>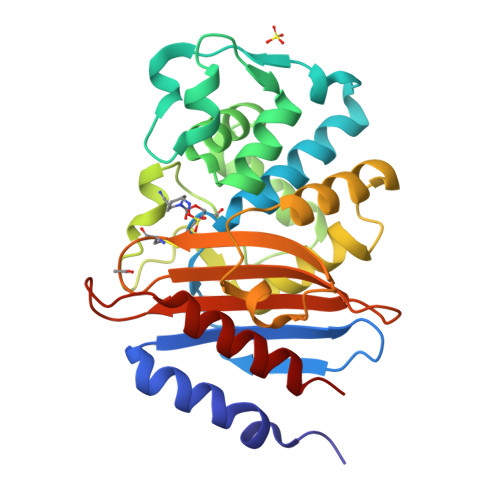ATALTNLVAEPFAKLEQDFGGSIGVYAMDTGSGATVSYRAEERFPLCSSFKGFLAAAVLARSQQQAGLLDTPIRYGKNALVPWSPISEKYLTTGMTVAELSAAAVQYSDNAAANLLLKELGGPAGLTAFMRSIGDTTFRLDRWELELNSAIPGDARDTSSPRAVTESLQKLTLGSALAAPQRQQFVDWLKGNTTGNHRIRAAVPADWAVGDKTGTCGVYGTANDYAVVWPTGRAPIVLAVYTRAPNKDDKHSEAVIAAAARLALEGLG[2x]>[3x]MPLDAGGQNSTQMVLAPGASIFRCRQCGQTISRRDWLLPMGGDHEHVVFNPAGMIFRVWCFSLAQGLRLIGAPSGEFSWFKGYDWTIALC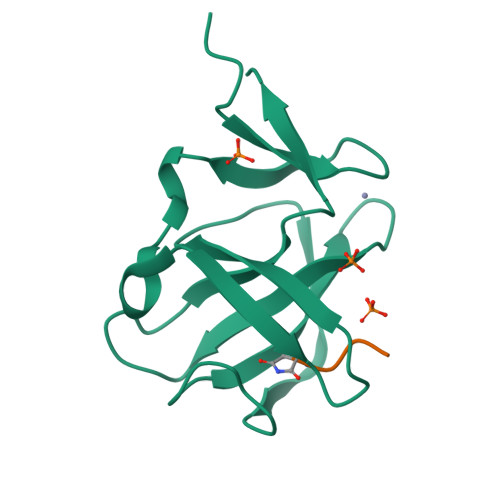GQCGSHLGWHYEGGSQPQTFFGLIKDRLAEGPAD;>QMQN[2x]> MGSSHHHH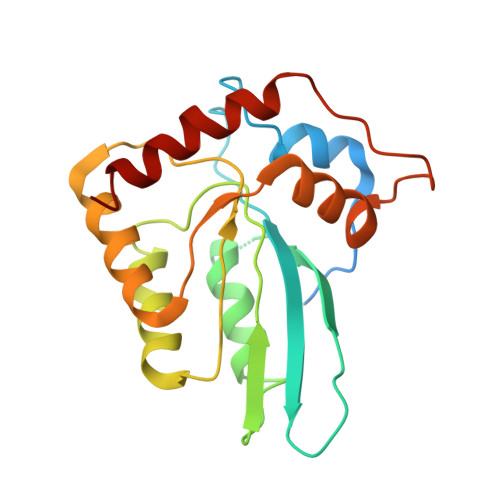HHSQDPNSMGKEILRNPMEAMDPHIFYFHFKNLRKAYGRNESWLCFTMEVVKHHSPVSWKRGVFRNQVDPETGRHAERCFLSWFCDDILSPNTNYEVTWYTSWSPCPECAGEVAEFLARHSNVNLTIKTARLYYFKDTDAAEGLRSLSQEGASVEIMGYKDFKYCWENFVYNDDEPFKPWDGLDYNFLDLDSKLQEILE> CUGCUGGCUAAGGCAUGAAAGUGCUAUGCCUGCUG

Our current understanding of the DM1 disease mechanism is that the CTG repeats are transcribed into toxic CUG-repeat RNA, which sequesters RNA-binding proteins that are important for gene regulation. The CUG repeats are toxic because they contain hundreds or thousands of YGCY motifs repeated in the expanded CUG repeats. Structure-probing, crystal and nuclear magnetic resonance structures have shown that CUG repeats can form double-stranded A-form helices (20–23). Pseudouridine (Ψ) is an isomerization product of uridine and is the most common RNA modification.

We previously utilized the GAAA tetraloop and its conserved 11 nucleotide receptor in order to facilitate the crystallization of CUG repeats (trCUG-3). In order to observe how Ψ affected the structure of CUG repeats, we substituted a Ψ in place of the U at position five in the trCUG-3 construct to create trCUG-3(Ψ5). The trCUG-3(Ψ5) construct readily crystallized and the structure was successfully solved using the trCUG-3 structure for molecular replacement (see Table 2 for data collection and refinement statistics). However, there were key differences when the U5–U31 base pair from the native structure was compared to the Ψ5–U31 base pair. Strikingly, there was a water molecule coordinating the amine group of Ψ5 to the carbonyl group of U31. Positions of the water and the non-canonical Ψ–U pair were confirmed by creating a simulated annealing omit map. In order to form these two additional hydrogen bonds, the Ψ5–U31 base pair has a greater opening angle compared to U5–U31 as well as a greater C1′–C1′ distance. This bridging water adds two additional hydrogen bonds between uridine and Ψ and may contribute to Ψ's structure-stabilizing capabilities in the context of CUG repeats.> MATGTRYAGKVVVVTGGGRGIGAGIVRAFVNSGARVVICDKDESGGRALEQELPGAVFILCDVTQEDDVKTLVSETIRRFGRLDCVVNNAGHHPPPQRPEETSAQGFRQLLELNLLGTYTLTKLALPYLRKSQGNVINISSLVGAIGQAQAVPYVATKGAVTAMTKALALDESPY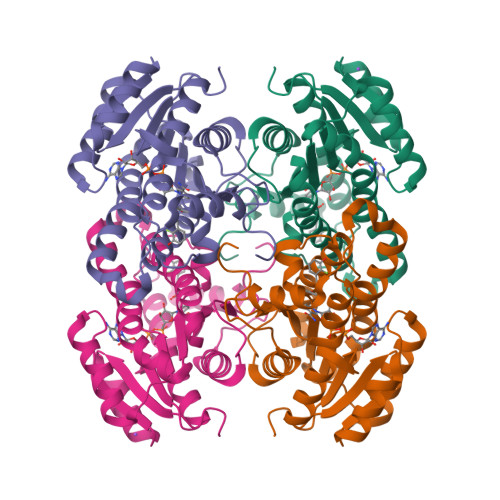GVRVNCISPGNIWTPLWEELAALMPDPRATIREGMLAQPLGRMGQPAEVGAAAVFLASEANFCTGIELLVTGGAELGYGCKASRSTPVDAPDIPS N-{5-[(4-ethylpiperazin-1-yl)methyl]pyridin-2-yl}-5-fluoro-4-[4-fluoro-2-methyl-1-(propan-2-yl)-1H-benzimidazol-6-yl]pyrimidin-2-amine 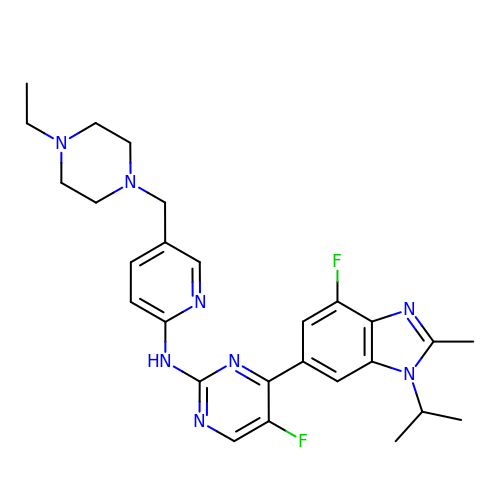| C27 H32 F2 N8 | UZWDCWONPYILKI-UHFFFAOYSA-N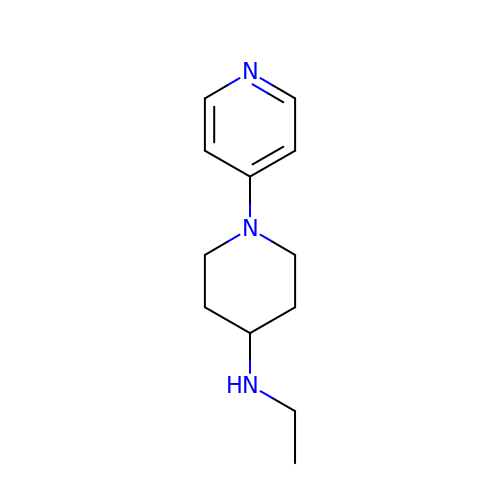N-ethyl-1-(pyridin-4-yl)piperidin-4-amine | C12 H19 N3 | SZIYLERKSNSGON-UHFFFAOYSA-N> AQTVPYGIPLIKADKVQAQGFKGANVKVAVLDTGIQASHPDLNVVGGASFVAGEAYNTDGNGHGTHVAGTVAALDNTTGVLGVAPSVSLYAVKVLNSSGSGSYSGIVSGIEWATTNGMDVINMSLGGASGSTAMKQAVDNAYARGVVVVAAAGNSGSSGNTNTIGYPAKYDSVIAVGAVDSNSNRASFSSVGAELEVMAPGAGVYSTYPTNTY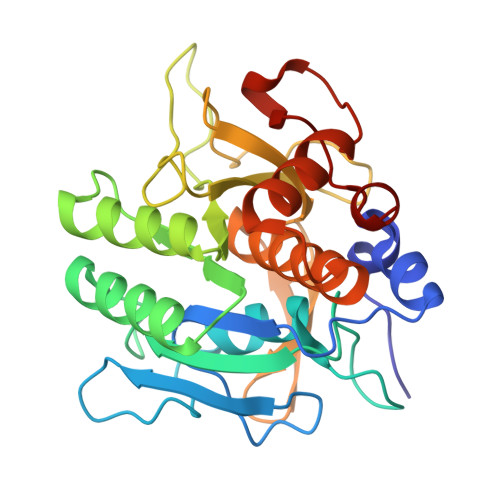ATLNGTSMASPHVAGAAALILSKHPNLSASQVRNRLSSTATYLGSSFYYGKGLINVEAAAQ>MVSLEKNDHLMLARQLPLKSVALILAGGRGTRLKDLTNKRAKPAVHFGGKFRIIDFALSNCINSGIRRMGVITQYQSHTLVQHIQRGWSFFNEEMNEFVDLLPAQQRMKGENWYRGTADAVTQNLDIIRRYKAEYVVILAGDHIYKQDYSRMLIDHVEKGARCTVACMPVPIEEASAFGVMAVDENDKIIEFVEKPANPPSMPNDPSKSLASMGIYVFDADYLYELLEEDDRDENSSHDFGKDLIPKITEAGLAYAHPFPLSCVQSDPDAEPYWRDV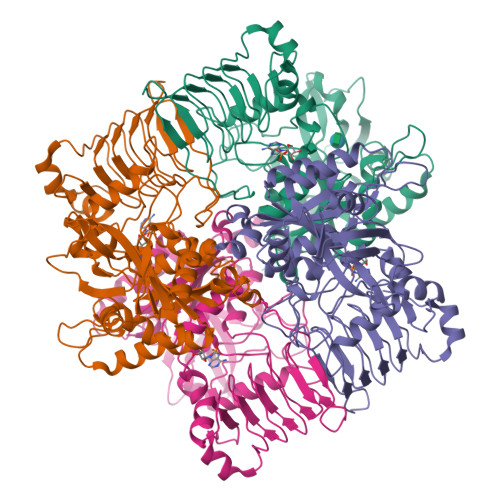GTLEAYWKANLDLASVVPELDMYDRNWPIRTYNESLPPAKFVQDRSGSHGMTLNSLVSGGCVISGSVVVQSVLFSRVRVNSFCNIDSAVLLPEVWVGRSCRLRRCVIDRACVIPEGMVIGENAEEDARRFYRSEEGIVLVTREMLRKLGHKQER[16x]> GSHMEMKKSGLGTTAIHAGTLKNLYGTLAMPIYQTSTFIFD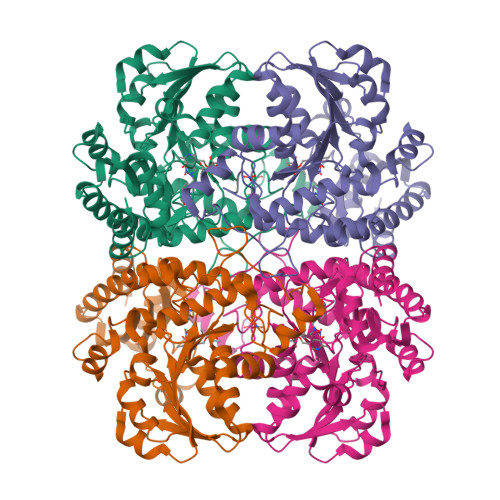SAEQGGRRFALEEAGYIYTRLGNPTTTVLENKIAALEEGEAGIAMSSGMGAISSTLWTVLKAGDHVVTDKTLYGCTFALMNHGLTRFGVEVTFVDTSNLEEVKNAMKKNTRVVYLETPANPNLKIVDLEALSKIAHTNPNTLVIVDNTFATPYMQKPLKLGVDIVVHSATKYLNGHGDVIAGLVVTRQELADQIRFVGLKDMTGAVLGPQEAYYIIRGLKTFEIRMERHCKNARTIVDFLNKHPKVEKVYYPGLETHPGYEIAKKQMKDFGAMISFELKGGFEAGKTLLNNLKLCSLAVSLGDTETLIQHPASMTHSPYTKEEREVAGITDGLVRLSVGLENVEDIIADLEQGLEKI>[6x]MADPSLNNPVVIQATRLDASILPRNVFSKSYLLYVIAQGTDVGAIAGKANEAGQGAYDAQVKNDEQDVELADHEARIKQLRIDVDDHESRITANTKAITALNVRVTTAEG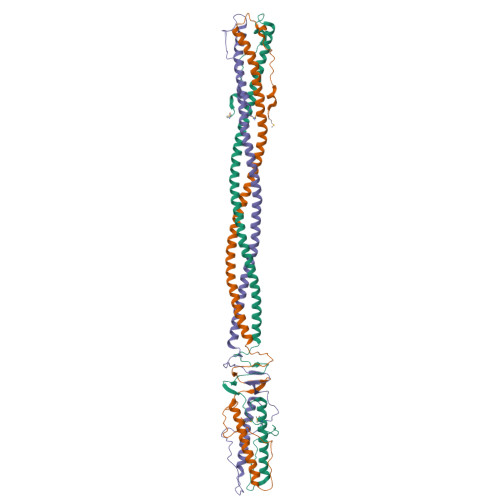EIASLQTNVSALDGRVTTAENNISALQADYVSKTATTSQSLASPLNVTTSYSVGGKKVVGARQTGWTAATGTANKGVFDADLTFAVSDTYTQSEIQAIANALITERRRTKAMEDALRAHGLID> MAEGSRGGPTCSGVGGRQDPVSGSGGCNFPEYELPELNTRAFHVGAFGELWRGRLRGAGDLSLREPPASALPGSQAADSDREDAAVARDLDCSLEAAAELRAVCGLDKLKCLEDGEDPEVIPENTDLVTLGVRKRFLEHREETITIDRACRQETFVYEMESHAIGKKPENSADMIEEGELILSVNILYPVIFHKHKEHKPYQTMLVLGSQKLTQLRDSIRCVSDLQIGGEFSNTPDQAPEHISKDLYKSAFFYFEGTFYNDKRYPECRDLSRTIIEWSESHDRGYGKFQTARMEDFTFNDLCIKLGFPYLYCHQGDCEHVIVITDIRLVHHDDCLDRTLY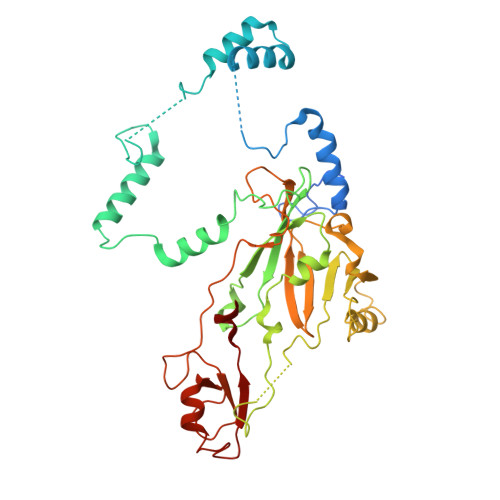PLLIKKHWLWTRKCFVCKMYTARWVTNNDSFAPEDPCFFCDVCFRMLHYDSEGNKLGEFLAYPYVDPGTFN>[2x]HMLEGGSGGSGGSTIYHAKDAVQATKPDMRKPRLVVFVVGETARADHVSFNGYERDTFPQLAKIDGVTNFSNVTSCGTSTAYSVPCMFSYLGADEYDVDTAKYQENVLDTLDRLGVSILWRDNNSDSKGVMDKLPKAQFADYKSATNNAICNTNPYNECRDVGMLVGLDDFVAANNGKDMLIMLHQMGNHGPAYFKRYDEKFAKFTPVCEGNELAKCEHQSLINAYDNALLATDDFIAQSIQWLQTHSNAYDVSMLYVSDHGESLGENGVYLHGMPNAFAPKEQRSVPAFFWTDKQTGITPMATDTVLTHDAITPTLLKLFDVTADKVKDRTAFIR

NDM-1, as a typical member of B1 class of MBLs, possesses two Zn(II) ions intercalated by a nucleophile hydroxide in its active site, which is delimited by flexible loop 3 and 1023. The two Zn(II) ions have been validated to be crucial for its hydrolytic activity to launch a nucleophilic attack on β-lactam rings in β-lactam antibiotics. The Zn(II) ion in the active site of MCR-1 has been validated to be vital for the PEA transfer process; notwithstanding its biological roles in MCR proteins are still controversial. Our results showed that AUR irreversibly inhibit NDM-1 activity and disrupted the function of MCR-1 via displacing Zn(II) ions in the active sites and thus forming Au-NDM-1 or Au-MCR-1.

Since AUR is a prodrug and metabolizes to an active species [Au(PEt3)]+ when transferred across cell membranes, we therefore used an AUR analogue, chloro(triethylphosphine)gold(I) [Au(PEt3)Cl], for all the enzyme-based biophysical studies to mimic its action in cellulo. The crystal structure of Au-MCR-1-S was resolved at 1.68 Å resolution and the binding of Au(I) to the MCR-1-S was also confirmed by X-ray excitation spectrum. From the density map, three Au ions were clearly visible in one chain in an asymmetric unit, and a single Au ion (Au542 with occupancy of 0.5) was found in the Zn-dependent catalytic core, coordinating with four residues, i.e., Glu246, Asp465, His466, and TPO285 to form a distorted tetrahedral geometry. The bond lengths of Au(I) with the side-chains of amino acid residues are overall slightly longer than those for Zn(II), probably owing to the larger ionic radius of Au(I) (1.37 Å) than Zn(II) (0.74 Å). The second Au ion (Au543) linearly coordinated to Nɛ2-His252 and PEt3 group (N–Au–P angle 171.5°). The third Au ion (Au544) coordinated to Nɛ2-His424 and a water molecule in a quasi-linear geometry (N–Au–O angle of 159.0°). The Au ion (Au543) was only observed in one chain in the asymmetric unit with occupancy of ~0.3, but not in the other one, inferring the less accessibility of Au(PEt3)Cl to this site. The crystallographic analysis demonstrates that AUR binds to MCR-1 and displaces Zn(II) in the active site through Au(I). We show that the Zn(II) ions in MCR-1 could be irreversibly kicked out by AUR and form an Au-bound MCR-1 with Au(I) coordinating to Glu246, Asp465, His466, and TPO285. Although there is no cysteine residues in the active site of MCR enzyme, to our surprise, unlike Bi(III) drugs, AUR also targets MCR-1 protein at its zinc-catalytic core through the side-chains (εN) of histidine residues, suggesting that the “softness” of histidine (e.g., εN) is tunable by a protein.Acetylcholine (ACh) is an important neurotransmitter in the central and peripheral nervous system where it mediates fast excitatory neurotransmission by binding to nicotinic acetylcholine receptors (nAChRs). A nAChR ligand-binding domain homologue, the ACh binding protein (AChBP), has proven a uniquely well-suited system for the study of receptor-ligand interactions. AChBP forms a pentameric structure where the interfaces between the subunits provide an ACh binding pocket that is homologous to the binding pocket of nAChRs. Ac-AChBP has so far been the most widely used for crystallization experiments; however, in the context of nAChRs the binding pocket of Ls-AChBP shows better resemblance as it contains all the five aromatic residues fully conserved in nAChRs.

Here, we report the crystal structure of ACh bound to Ls-AChBP. A complete data set was collected to 2.6 Å resolution and the asymmetric unit of the crystal contains two pentamers, corresponding to a total of 2024 residues built. Additional electron density for a single ACh molecule was present at all ten subunit interfaces. The ligand adopts a similar location and conformation (average RMSD of 0.04 Å between all ACh non-hydrogen atoms) at each interface and binds under a closed loop C. The C loops have a uniform degree of closure across the interface (∼7.7 Å) when measured from the disulphide bridge (C atom of Cys187) to the backbone carbonyl oxygen atom of Trp143. The ligand-protein interactions are characterized by contacts to an aromatic box formed primarily by residues on the principal side of the interface (residues Tyr89, Trp143, Tyr185 and Tyr192) but also by Trp53 on the complementary side. The backbone carbonyl oxygen atom of Trp143 interacts with the carbon adjacent to the ammonium group of ACh at a distance of 3.1 Å (3.0–3.2 Å), similar to a previous observation for carbamoylcholine. The anchoring to this side is characterized by a binding site water molecule located 3.5 Å (3.3–3.6 Å) from the carbonyl oxygen atom of ACh. In addition to the water-mediated hydrogen bonds, Trp53 is positioned to interact with the trimethylammonium group of ACh with a distance of 4.9 Å (distance between trimethylammonium nitrogen of ACh and the centroid of the benzene part of the indole in the tryptophan side chain: 5.8 Å (5.4–6.1 Å)), i.e. within the 6 Å that has been used as a rough limit when identifying cation-π interactions. At four binding sites, a PEG400 molecule from the crystallization buffer is located within 4.5 Å of ACh. Apparently without affecting the binding mode of ACh in a direct manner, when these PEG400 molecules are present Trp53 adopts a conformation pointing deeper into the binding site (light blue and Figure 3C).

>[10x]MRRNIFCLACLWIVQACLSLDRADILYNIRQTSRPDVIPTQRDRPVAVSVSLKFINILEVNEITNEVDVVFWQQTTWSDRTLAWNSSHSPDQVSVPISSLWVPDLAAYNAISKPEVLTPQLARVVSDGEVLYMPSIRQRFSCDVSGVDTESGATCRIKIGSWTHHSREISVDPTTENSDDSEYFSQYSRFEILDVTQKKNSVTYSCCPEAYEDVEVSLNFRKKGRSEIL>[4x]MSARRTESDIQGFHATPEFGGNL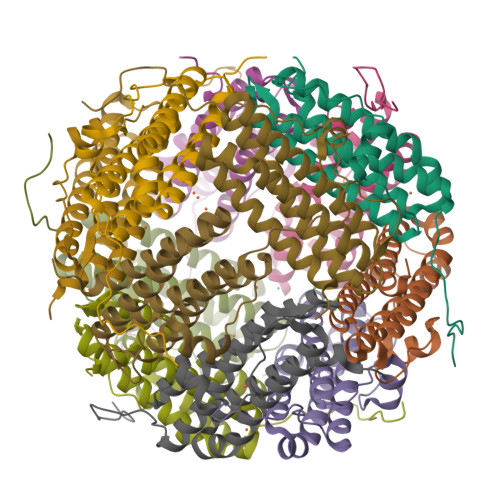QKVLVDLIELSLQGKQAHWNVVGSNFRDLHLQLDELVDFAREGSDTIAERMRALDAVPDGRSDTVAATTTLPEFPAFERSTADVVDLITTRINATVDTIRRVHDAVDAEDPSTADLLHGLIDGLEKQAWLIRSENRKV>[2x]TEDERRELEKVARKAIEAAREGNTDEVREQLQRALEIARESGSEEAFKLALEVVRRVAEVAARAGNVEAVKEALRVALEIVKEAMELIKDPEAIVRLALEAVRVVAEVA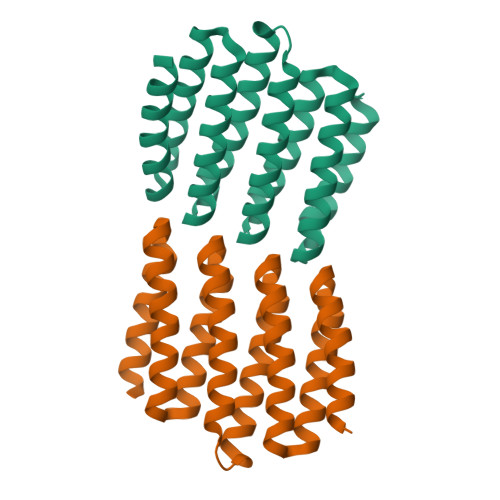ARAGAVEAVKVALRVALEIAKIAGTEEAVRLALEVVKRVSDIAKKAGNEDAVKEAEEVRKKIEEESGGSGSHHWGSTHHHHHH The Myxococcus xanthus FrzS protein transits from pole-to-pole within the cell, accumulating at the pole that defines the direction of movement in social (S) motility. The N-terminal receiver domain (RD), a 258-residue coiled-coil domain, and the extreme C-terminal tail of the protein are all required for the dynamic subcellular localization and S-motility activity of FrzS. Here we show using atomic-resolution crystallography and NMR that the FrzS receiver domain (RD) displays the conserved switch Tyr102 in an unusual conformation, lacks the conserved Asp phosphorylation site, and fails to bind Mg2+ or the phosphoryl analogue, Mg2+·BeF3. The crystal structures of the mutants suggested that the observed conformation of Tyr102 in the wild-type FrzS RD is not sufficient for function. These results support the model that FrzS contains a novel ‘pseudo-receiver domain’ whose function requires recognition of the RD output face but not Asp phosphorylation.

To test whether the environment of Tyr102 is important for domain function, we mutated His92, which forms a hydrogen bond to the buried Tyr102 hydroxyl group in the FrzS RD structure, to a phenylalanine. The His92Phe mutation blocked social motility to the same extent as the Tyr102Ala mutation with no effect on protein stability. The His92Phe mutant crystallized in a distinct monoclinic space group (P21), with one crystal contact within 4 Å of the α4-β5-α5 output face, as quantified by the Crystal Contacts Analysis Server. In total, the intermolecular contact area decreased from an average of 4806 Å2/RD-monomer in the hexagonal crystals to 1594 Å2/monomer in the monoclinic His92Phe RD crystals. The His92Phe replacement was expected to cause the Tyr102 side chain to switch to the outward facing rotamer due to the increased volume of Phe and the loss of the hydrogen bond between Tyr102 and the His92 side chains. Unexpectedly, Tyr102 remained facing inward in the structure of the His92Phe variant, and the Phe92 side chain shifted away from Tyr102. The overall Cα RMSD for the His92Phe variant and hexagonal wild-type RD structures was 0.35 Å. In summary, the His92Phe RD structure is nearly identical to the hexagonal wild-type RD structure in both the dynamic β3-α3 loop and the output face of the RD. The similarly inactivating His92Phe mutation, however, preserved the conformation of Tyr102 in the crystal structure of the mutant protein. Rather, the His92Phe mutation may compromise an alternative conformation of the α4-β5-α5 face or interrupt a signalling pathway required to switch the conformation of Tyr102 and to retain FrzS at the leading pole during S-motility.

> GSHMSKKILIVESDTALSATLRSALEGRGFTVDETTDGKGSVEQIRRDRPDLVVLAVDLSAGQNGYLICGKLKKDDDLKNVPIVIIGNPDGFAQFRKLKAHADEYVAKPVDADQLVERAGALIGFPE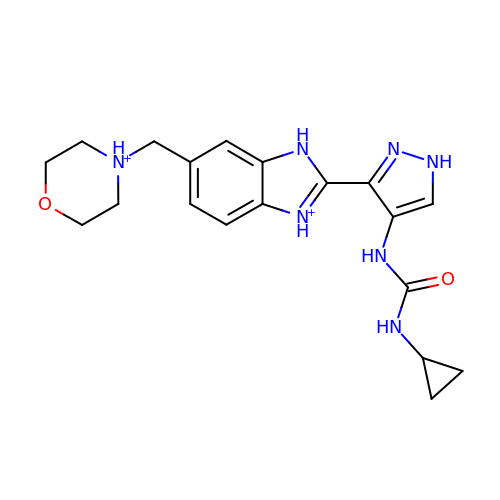2-{4-[(CYCLOPROPYLCARBAMOYL)AMINO]-1H-PYRAZOL-3-YL}-6-(MORPHOLIN-4-IUM-4-YLMETHYL)-1H-3,1-BENZIMIDAZOL-3-IUM | C19 H25 N7 O2 | LOLPPWBBNUVNQZ-UHFFFAOYSA-P Cyclodipeptide synthases (CDPSs) use aminoacylated tRNA (aa-tRNA) substrates to form peptide bonds between two amino acids yielding a cyclic dipeptide product (CDP). ParaCDPS from Parabacteroides sp. 20_3 (GenBank: EFK64745.1) produces cyclo(His-Phe)8 whilst ParcuCDPS from Parcubacteria bacterium RAAC4_OD1_1 (GenBank: ETB63777.1) can synthesise both cyclo(His-Glu) and cyclo(His-Pro)9. ParcuCDPS belongs to the XYP sub-group of the CDPS family, characterised by the presence of 3 residues: X40 where X is a non-conserved residue, Y202, and P203 (numbering respective to AlbC). ParcuCDPS displays a Rossman-fold common throughout the CDPS family.

Inspired by HisRS and histidine recognition more generally, and by the only high resolution structure of a CDPS with a ligand bound, we systematically altered three unique residues in ParcuCDPS P1, which we hypothesised to be participating in crucial interactions with the polar side chain of histidine. We first designed Generation 1 containing seven P1 mutants (Y55F; Y55V; E174A; E174H; E174L; Y189F and Y189L), and these variants were cloned, expressed in E.coli, purified and used for activity assays. By mutating the P1 residues, the activity of the variants was vastly reduced with E174A and E174H incapable of tolerating histidine as a substrate. The impact of mutating Y55 carries more weight than Y189, suggesting it may directly interact with the histidine residue via a H-bond rather than adding to the polar surface. A similar pattern of residues interacting with the imidazole from histidine is seen in HisRS, in which two tyrosine and a glutamate residue mediate interactions with the nitrogen groups of histidine. Further investigation into the changes imposed by these mutants was performed by solving the crystal structures of a select few mutants containing changes to the active site or the pocket residues. The mutant structures were able to be solved using WT as a model and retained an equivalent fold to ParcuCDPS (Supplementary Notes 4 and 7 relating to Supplementary Figs. 13 and 14). Therefore, the disruption of activity is caused exclusively by the change in these few residues which appear important for the enzyme to produce a CDP.

> MELHQIRGCHKNDIELKKYNIGVAISLGNKWFSIDNIEKLVKWSLLHTKEYVIIFIADSIHGINLSVRNKLSDSHAEEVAIRYGRNLFIKIKERVSLSFSQDEQAKIIYATWSDIADSKYKEKVKYLYNLYDKNINFKNYIENFVKEWVSKEKRTFNNNEINKFGRYILEELPELMVQVKARGVLFEAYVYPYKTRITEFVGLLQKGEIFPEIKTNILDNHPKIFLEVREHHHHHH[(8S)-8-(chloromethyl)-7,8-dihydro-6H-furo[3,2-e]indol-6-yl](5-fluoro-1H-indol-2-yl)methanone | C20 H14 Cl F 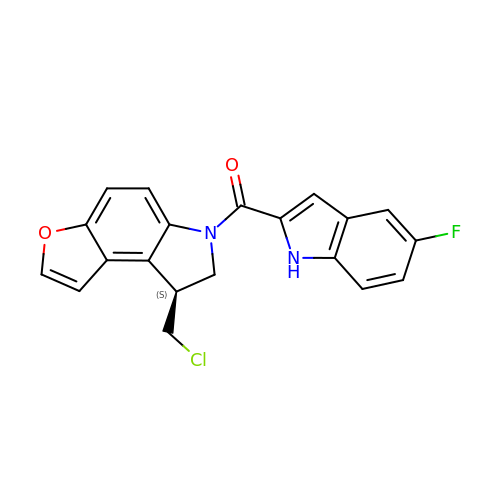N2 O2 | ATYWMISRLWKSNW-GFCCVEGCSA-N> SQPIFLNVLEAIEPGVVCAGHDNNQPDSFAALLSSLNELGERQLVHVVKWAKALPGFRNLHVDDQMAVIQYSWMGLMVFAMGWRSFTNVNSRMLYFAPDLVFNEYRMHKSRMYSQCVRMRHLSQEFGWLQITPQEFLCMKALLLFSIIPVDGLKNQKFFDELRMN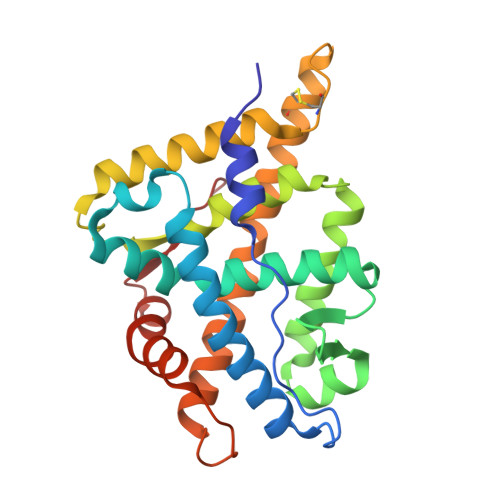YIKELDRIIACKRKNPTSCSRRFYQLTKLLDSVQPIARELHQFTFDLLIKSHMVSVDFPEMMAEIISVQVPKILSGKVKPIYFHT>MGSSHHHHHHSSGRE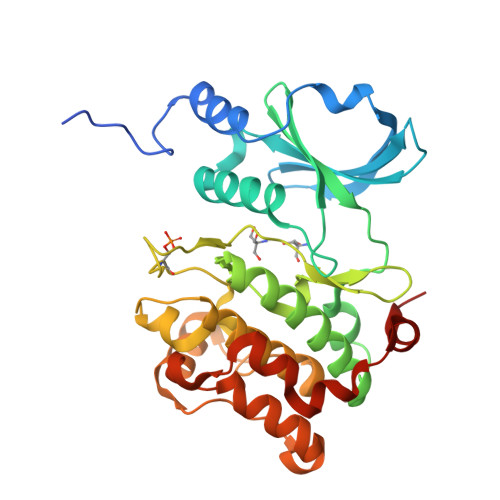NLYFQSMSRVSHEQFRAALQLVVSPGDPREYLANFIKIGEGSTGIVCIATEKHTGKQVAVKKMDLRKQQRRELLFNEVVIMRDYHHDNVVDMYSSYLVGDELWVVMEFLEGGALTDIVTHTRMNEEQIATVCLSVLRALSYLHNQGVIHRDIKSDSILLTSDGRIKLSDFGFCAQVSKEVPKRKSLVGTPYWMAPEVISRLPYGTEVDIWSLGIMVIEMIDGEPPYFNEPPLQAMRRIRDSLPPRVKDLHKVSSVLRGFLDLMLVREPSQRATAQELLGHPFLKLAGPPSCIVPLMRQYRHH[2x]RepB, the replication initiation protein of pMV158, is a member of the HUH endonuclease superfamily, which includes proteins involved in the replication of plasmids, bacteriophages and viruses, as well as proteins with roles in DNA transposition and in conjugative mobilisation of plasmids. These proteins are characterised by the presence of two conserved protein motifs: the HUH motif, composed of two His residues separated by a bulky hydrophobic amino acid, which is responsible for the coordination of a divalent metal cation, and the catalytic motif, containing one or two Tyr residues separated by several amino acids. Each monomer of RepB comprises two domains connected by a short hinge region. The C-terminal or oligomerisation domain (OD) is a helical domain responsible for the hexameric state of the protein, while the N-terminal or origin binding domain (OBD) carries the catalytic active site and is in charge of recognising, cleaving and joining dso DNA.

A new crystal structure for the RepB hexamer was obtained without DNA in the crystallisation conditions. However, the most striking feature of this new structure is the prolongation of α5 helix by two turns, expanding to the region connecting the ODs and OBDs, in two of the protomers (chains B and D), in place of the 310-helix and the flexible region (residues 128–153) observed in the previous hexameric structures and in the remaining protomers of the current structure. Alignment through the OD region of protomers with this extended helix (chains B or D) against a protomer with a flexible region (i.e. chain A) shows a large anticlockwise rotation of the OBD of almost 180° relative to the OD. As a result of this new arrangement, the OBD of these two chains is positioned over the OBD of the neighbouring protomers, chains C and E, respectively, thereby occluding access to the active site of protomers B and D within the structure and impeding the cleavage activity on the nick site. Therefore, these two protomers must be inactive within this hexamer conformation. Another consequence of the presence of a longer α5 helix in two of the monomers is that the neighbouring subunits (protomers C and E) also present a dramatic change of orientation of the OBD relative to the OD. Since the OBD of chains B and D are in such immediacy to those of subunits C and E, respectively, the active sites of the latter are forced to move closer to the OD and face it, instead of being exposed at the top of the cup-shaped hexamer. The α2 helix faces the outer circumference of the hexamer in subunits B, C, D and E, instead of being exposed at the top of the cup, as in the case of the other two chains, A and F, and in all the protomers of the two structures previously reported. A phosphate molecule bound to the active site is observed in all the subunits of this new hexamer, instead of the catalytic Mn2+ metal ion reported in the other two hexamers.

>[6x]MAKEKARYFTFLLYPESIPSDWELKLETLGVPMAISPLHDKDKSSIKGQKYKKAHYHVLYIAKNPVTADSVRKKIKLLLGEKSLAMVQVVLNVENMYLYLTHESKDAIAKKKHVYDKADIKLINNFDIDRYVTLDVEEKTELFNVVVSLIRAYTLQNIFDLYDFIDENGETYGLTINLVNEVIAGKTGFMKLLFDGAYQRSKRGTKNEER>MAHHHHHHMLKETYPYYLANEAVYANAELEVTDKYTGKVATRVALADASAIDAAIAAAVGAQKPLRALPAFRRQAILEHCVARFRERFDELAQALCIEAGKPINDSKGEVTRLIDTFRVAAEESVRIEGGLVNLEISPRAQGYSGYYKRVPIGPCSFISPFNFPLNLAAHKVAPALAAGCPFVLKPASRTPIGALIIGEVLAETDLPKGAFSILPAHRDGADLFTTDERFKLLSFTGSPTVGWELKKKAGKKKVVLELGGNAAAIVDADQREVLDYVVERLAFGAYYQSGQSCIGVQRIIAHADVYDALREKLIAKTRSLKMGDPKDPATFVGPMISESEARRLAGWMEAAVAAGAKIVAGGKVDGA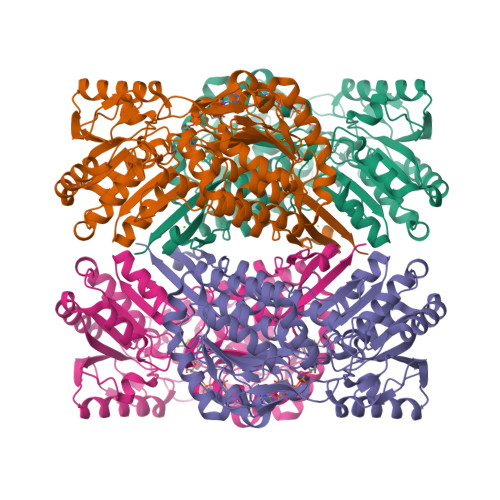MFEATLLEGVGRDQDLYRKEAFGPVALLERFSDFDDALARVNDSDFGLQAGVFTDSLSHAQRAWDELEVGGVVINDVPSFRVDNMPYGGVKDSGLGREGIRYAIEDMTELRLMVVRRR[4x]> MKRVMFHAKIHRATVTQADLHYVG;> VTVDQDLLDAAGILPFEQVDIYDITNGARLTTYALPGERGS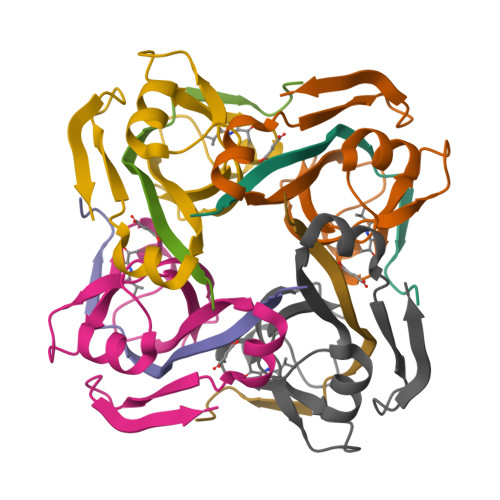GVIGINGAAAHLVKPGDLVILVAYGVFDEEEARNLKPTVVLVDERNRILEVRKG> DVQPETCRPSAASGNYFPQYPEYAIETARLRTFEAWPRNLKQKPHQLAEAGFFYTGVGDRVRCFSCGGGLMDWNDNDEPWEQHALWLSQCRFVKLMKGQLYIDTVAAKPV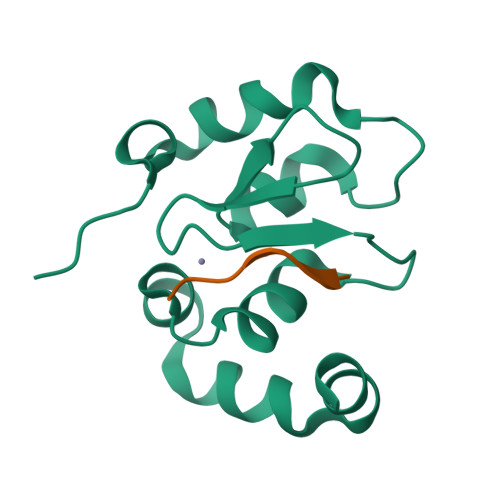LAEEKEESTSIGGD;> AVPFYLPEGG> ACVHHIKRRDIVLKWELGEGAFGKVFLAECHNLLPEQDKMLVAVKALKEASESARQDFQREAELLTMLQHQHIVRFFGVCTEGRPLLMVFEYMRHGDLNRFLRSHGPDAKLLAGGEDVAPGPLGLGQLLAVASQVAAGMVYLAGLHFVHRDLATRNCLVGQGLVVKIGDFGMSRDIYSTDYYRVGGRTMLPIRWMPPESILYRKFTTESDVWSFGVVLWEIFTYGKQPWYQLSNTEAIDCITQGRELERPRACPPEVYAIMRGCWQREPQQRHSIKDVHARLQ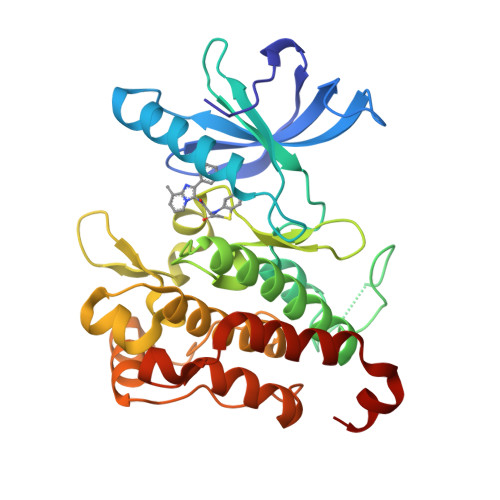ALAQAPPVYLDVLG>[2x]ALYEDPPDQKTSPSGKPATLKICSWNVDGLRAWIKKKGLDWVKEEAPDILCLQETKCSENKLPAELQELPGLSHQYWSAPSDKEGYSGVGLLSRQAPLKVSYGIGDEEHDQEGRVIVAEFDSFVLVTAYVPNAGRGLVRLEYRQRWDEAFRKFLKGLASRKPLVLCGDLNVAHEEIDLRNPKGNKKNAGFTPQERQGFGELLQAVPLADSFRHLYPNTPYAYTFWTYMMNARSKNVGWRLDYFLLSHSLLPALCDSKIRSKALGSDHCPITLYLAL

Human APE1 is an essential enzyme and multifunctional nuclease with AP-endonuclease, 3′ phosphodiesterase, 3′ to 5′ exonuclease, and RNA cleavage activities. Instead, rAPs are processed by AP-Endonuclease 1 (APE1), a multifunctional enzyme in the base excision repair (BER) pathway. During BER, abasic (AP) sites are first processed by APE1, which cleaves 5′ of the abasic site generating 3′ hydroxyl and 5′ deoxyribose phosphate termini. Here, we utilize enzyme kinetics, X-ray crystallography, and molecular dynamics simulations to provide insight into rAP processing by APE1.

To further probe the role of the catalytic metal, we solved additional rAP:APE1 complex structures in the presence of MnCl2. Using this approach, we were able to obtain both substrate and product crystals with Mn2+ bound within the APE1 active site, which diffracted to 2.57 and 2.00 Å, respectively. One advantage of using Mn2+ in crystallography is that its position in the structure can be validated by identifying its anomalous signal. In the rAP product structure, Mn2+ sits in the metal binding pocket, overlaying with the Mg2+ of the deoxy-AP structure, and coordinated by E96, D70, D308. Since both the Mn2+ metal ion and the 5′ phosphate cannot simultaneously occupy this pocket, the phosphate group of the rAP has shifted out of the pocket in the Mn2+ bound structure, where it now overlays with the position of 5′ phosphate in the deoxy-AP structure. This shift, compared to the non-metal bound structure, places the phosphate group in position to be coordinated by the same residues as the deoxy product (N174, N212, D210, Y171, H309). In addition to this main conformation, a second conformation was identified in the Mn2+ bound rAP product structure at only 25% occupancy. In the second conformation, the rAP phosphate is shifted into the metal binding pocket, as seen in the non-metal bound product structure, again highlighting the conflict that exists between the metal and the phosphate group. The existence of two alternate conformations of the nicked rAP site in this structure resulted in globular density that prevented accurate determination of the sugar pucker. Together, this data suggests that the APE1 catalytic metal helps to organize the APE1 active site during cleavage of an abasic ribonucleotide embedded in DNA.>[2x]GSTAPPTNQWYHGKLDRTIAEERLRQAGKSGSYLIRESDRRPGSFVLSFLSQMNVVNHFRIIAMSGDYYIGGRRFSSLSDLIGYYSHVSSLLKGEKLLYPVAPPEPVEDRRRVRAILPYTKVPDTDEISFLKGDMFIVHNELEDGWMWVTNLRTDEQGLIVEDLVEEVGREEDPHEGKIWFHGKISKQEAYNLLMTVGQVSSFLVRPSDNTPGDYSLYFRTNENIQRFKISPTPNNQFMM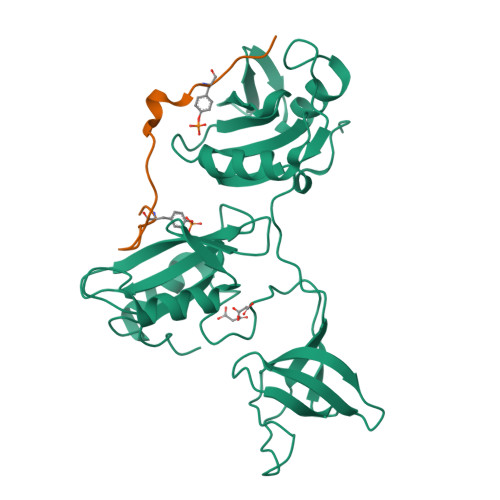GGRYYNSIGDIIDHYRKEQIVEGYYLKEPVPMQ;>DPSDYAEPMDAVVKPRNEEENIYSVPHDS[2x]>[4x]GPHMGGSMEALIPVINKLQDVFNTVGADIIQLPQIVVVGTQSSGKSSVLESLVGRDLLPRGTGIVTRRPLILQLVHVSQEDKRKTTGEENGVEAEEWGKFLHTKNKLYTDFDEIRQEIENETERISGNNKGVSPEPIHLKIFSPNVVNLTLVDLPGMTKVPVGDQPKDIELQIRELILRFISNPNSIILAVTAANTDMATSEALKISREVDPDGRRTLAVITKLDLMDAGTDAMDVLMGRVIPVKLGIIGVVNRSQLDINNKKSVTDSIRDEYAFLQKKYPSLANRNGTKYLARTLNRLLMHHIRDCLPELKTRI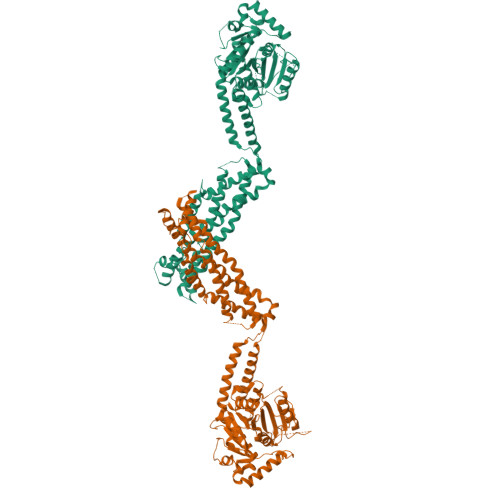NVLAAQYQSLLNSYGEPVDDKSATLLQLITKFATEYCNTIEGTAKYIETSELCGGARICYIFHETFGRTLESVDPLGGLNTIDILTAIRNATAAAAALFVPEVSFELLVKRQIKRLEEPSLRCVELVHEEMQRIIQHCSNYSTQELLRFPKLHDAIVEVVTCLLRKRLPVTNEMVHNLVAIELAYINTKHPDFADACGLMNNNIEEQRDCEVIERLIKSYFLIVRKNIQDSVPKAVMHFLVNHVKDTLQSELVGQLYKSSLLDDLLTESEDMAQRRKEAADMLKALQGASQIIAEIRETHLW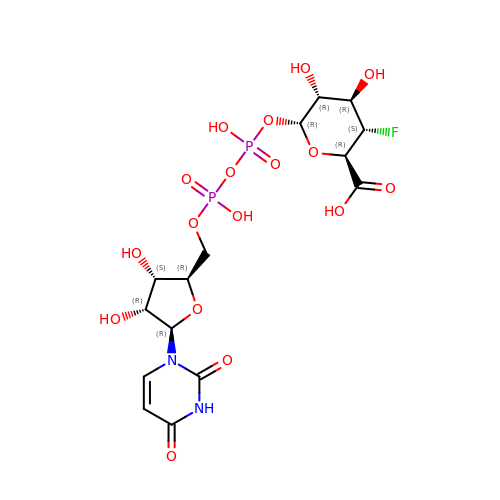(2~{R},3~{S},4~{R},5~{R},6~{R})-6-[[[(2~{R},3~{S},4~{R},5~{R})-5-[2,4-bis(oxidanylidene)pyrimidin-1-yl]-3,4-bis(oxidanyl)oxolan-2-yl]methoxy-oxidanyl-phosphoryl]oxy-oxidanyl-phosphoryl]oxy-3-fluoranyl-4,5-bis(oxidanyl)oxane-2-carboxylic acid | C15 H21 F N2 O17 P2 | LVBLRZZISSCAOI-CTMYAEKBSA-N5-[(4-METHYLPHENYL)SULFANYL]-2,4-QUINAZOLINEDIAMINE | C15 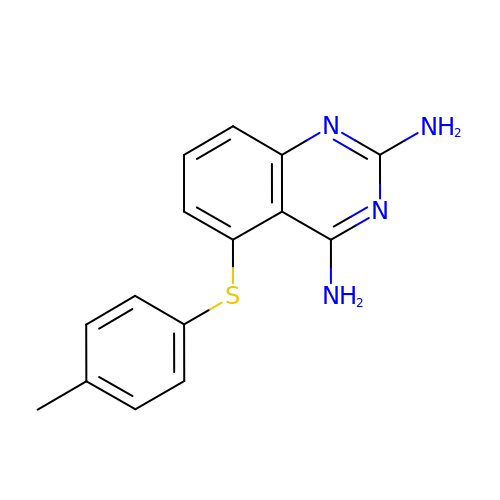H14 N4 S | UOJFGEAPSYQDIP-UHFFFAOYSA-N> QNVQHQLAQFQQLQQQAQAISVQKQTVEMQINETQKALEELSRAADDAEVYKSSGNILIRVAKDELTEELQEKLETLQLREKTIERQEERVMKKLQEMQVNIQEAMK;> NVQHQLAQFQQLQQQAQAISVQKQTVEMQINETQKALEELSRAADDAEVYKSSGNILIRVAKDELTEELQEKLETLQLREKTIERQEERVMKKLQEMQVNIQEA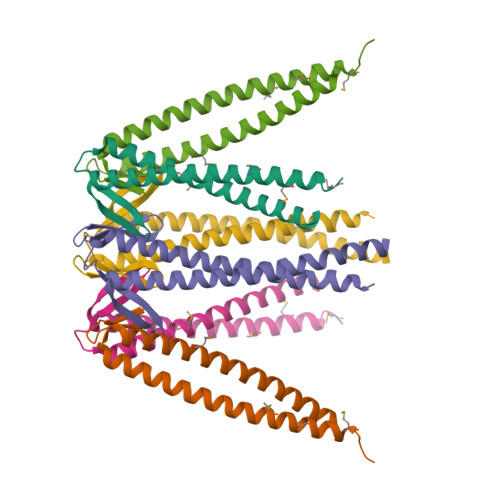MKGAG;> AALAEIVAQLNIYQSQVELIQQQMEAVRATISELEILEKTLSDIQGKDGSETLVPVGAGSFIKAELKDTSEVIMSVGAGVAIKKNFEDAMESIKSQKNELESTLQKMGENLRAITDIMMKLSPQAEELLAAVA> MGSSHHHHHQENLYFQSGPDEAKIKALLERTGYTLDVTTGQRKYGGPPPDSVYSGVQPGIGTEVFVGKIPRDLYEDELVPLFEKAGPIWDL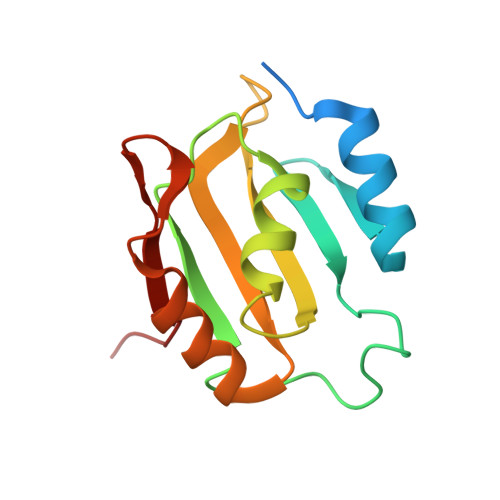RLMMDPLSGQNRGYAFITFCGKEAAQEAVKLCDSYEIRPGKHLGVCISVANN>[7x]NVKTIAHWVQ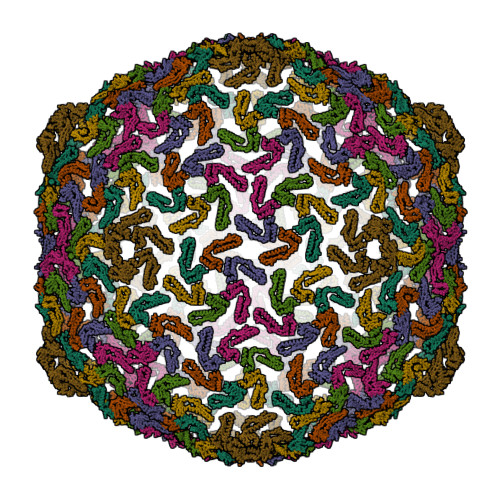ASRQVMDDAPMLQSYINNRLMYGLALKEEGQLLNGDGTGDNLEGLNKVATAYDTSLNATGDTRADIIAHAIYQVTESEFSASGIVLNPRDWHNIALLKDNEGRYIFGGPQAFTSNIMWGLPVVPTKAQAAGTFTVGGFDMASQVWDRMDATVEVSREDRDNFVKNMLTILCEERLALAHYRPTAIIKGT>[2x]MGVDPFQVAVGVSNRHIHLSRTDMDTLFGPGAELQRKKAMKQPGQFAAEETVTLKGPKGSLSKVRVLGPLRRETQVEVSVADGFALGITPPLR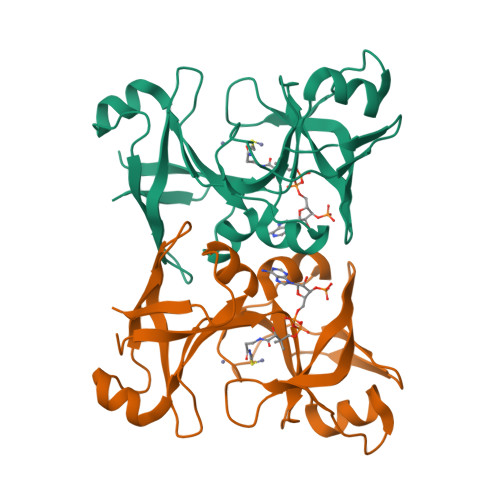QSGQLDDTPGLTIIGPQGSVTKDHGVIVAQRHIHMHPSTAAKLGLRNGDEVDVEAGGERGGVMHRVLIRVAEASADEMHIDVEEANALCLKNDDVVRICKKLEHHHHHH> LNRQVTVQRKEKDFQGMLEYHKEDEALLIRNLVTDLKPQMLSGTVPCLPAYILYMCIRHADYTNDDLKVHSLLTSTINGIKKVLKKHNDDFEMTSFWLSNTCRLLHCLKQYSGDEGFMTQNTAKQNEHCLKNFDLTEYRQVLSDLSIQIYQQLIKIAEGVLQPMIVSAMLENESIQGLSGVKPTGYRKRSSSMADGDNSYCLEAIIRQMNAFHTVMCDQGLDPEIILQVFKQLFYMINAVTLNNLLLRKDVCSWSTGMQLRYNISQLEEWLRGRNLHQSGAVQTMEPLIQAAQLLQLKKKTQEDAEAICSLCTSLSTQQIVKILNLYTPLNEFEERVTVAFIRTIQAQLQERNDPQQLLLDAKHMFPVLFPF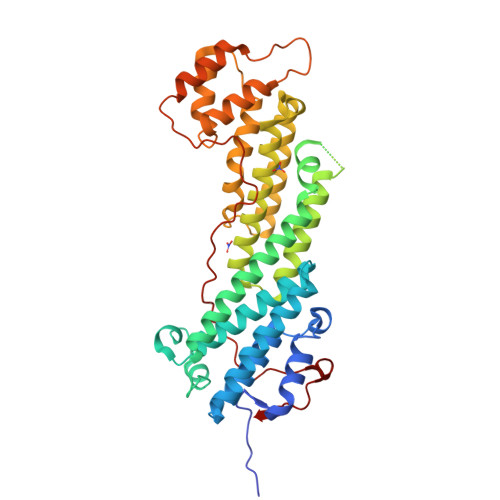NPSSLTMDSIHIPACLNLEFLNEV>GASIFRCRQCGQTISRRDWLLPMGGDHEHVVFNPAGMIFRVWCFSLAQGLRLIGAPSGEFSWFKGYDWTIALCGQCGSHLGWHYEGGSQPQTFFGLIKDRLAEGPA[3x]

Nowadays, the E3 ligase substrate receptor cereblon (CRBN), thalidomide’s primary target, is of particular importance in the fields of MGs and PROTACs. However, these CRBN ligands induce the degradation of IMiD neosubstrates and are inherently unstable, degrading hydrolytically under moderate conditions. In this work, we simultaneously optimized physiochemical properties, stability, on-target affinity, and off-target neosubstrate modulation features to develop novel nonphthalimide CRBN binders. These efforts led to the discovery of conformationally locked benzamide-type derivatives that replicate the interactions of the natural CRBN degron, exhibit enhanced chemical stability, and display a favorable selectivity profile in terms of neosubstrate recruitment.

Halo derivatives 8d (R = F) and 11a (R = Cl) could benefit from both mechanisms, haloalkyl compound 11b (R = CF3) displays strong deactivating properties, whereas compounds 11c (R = CH3), 11d (R = OMe), and 11e (R = OH) have ascending electron donating features. In addition, 11d and 11e could contribute to IMHBs. Fortunately, we could study all compounds generated in this iterative step through cocrystal structures in complex with the hTBD homolog MsCI4.44 These data confirmed that the preferred orientation of the ortho substituent toward the amide NH was preserved in the bound state of all ligands except for 11b. Sub van der Waals distances ranging from 1.3 to 2.0 Å were seen in 8d, 11a, 11c, 11d, 11e, and 11f. Hit compound 11e had to be excluded from further development due to the formation of reactive oxygen species (ROS) in the presence of the reducing agent tris(2-carboxyethyl)phosphine (TCEP). Subsequently, the aqueous stability was determined spectrophotometrically by following the changes in the absorption spectra of the compounds at pH 7.0, 8.0, and 9.0. These data confirmed the known hydrolytic susceptibility of compound 2,14,24 and revealed poor stability of 11e at higher pH values. Encouragingly, even compounds with CRBN binding affinity similar to lenalidomide, such as 11d and 11e, did not trigger substantial degradation of SALL4.>[4x]GGSMSNPDYCIPNFSQTVNERTIIDIFTICRYRSPLVVFCLSHNELAKKYAQDVSMSSGTHVHIIDGSVEITVSLYRTFRTIATQLLGRMQIVVFVTVDKSVVSTQVMKSIAWAFRGSFVELRNQSVDSSTLVSKLENLVSFAPLYNVPKCGPDYYGPTVYSELLSLATNARTHWYATIDYSMFTRSVLTGFVAKYFNEEAVPIDKRIVSIVGYNPPYVWTCLRHGIRPTYIEKSLPNPGGKGPFGLILPVINELVLKSKVKYVMHNPQIKLLCLDTFMLSTSMNILYIGAYPAT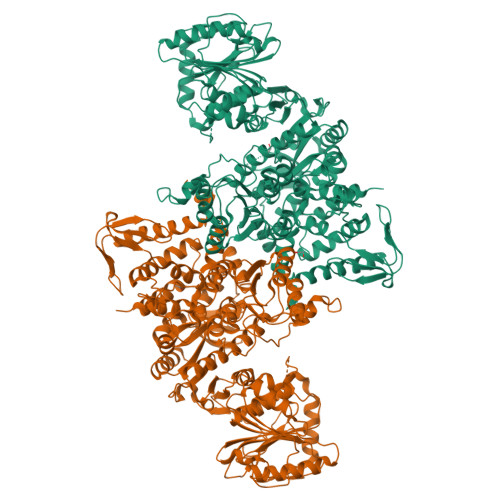HLLSLQLNGWTILAFDPKITSDWTDAMAKATGAKVIGVSKEFDFKSFSVQANQLNMFQNSKLSVIDDTWVETDYEKFQSEKQAYFEWLIDRTSIDVRLISMKWNRSKDTSVSHLLALLPQPYGASIREMRAFFHKKGASDIKILAAETEKYMDDFTAMSVSDQINTQKFMHCMITTVGDALKMDLDGGRAVIASYSLSNSSNSKERVLKFLSDANKAKAMVVFGAPNTHRLAYAKKVGLVLDSAIKMSKDLITFSNPTGRRWRDYGYSQSELYDAGYVEITIDQMVAYSSDVYNGVGYFANSTYNDLFSWYIPKWYVHKRMLMQDIRLSPAALVKCFTTLIRNICYVPHETYYRFRGILVDKYLRSKNVDPSQYSIVGSGSKTFTVLSHFEVPHECGPLVFEASTDVNISGHLLSLAIAAHFVASPMILWAEQMKYMAVDRMLPPNLDKSLFFDNKVTPSGALQRWHSREEVLLAAEICESYAAMMLNNKHSPDIIGTLKSAINLVFKI> MAAAVAMETDDAGNRLRFQLELEFVQCLANPNYLNFLAQRGYFKDKAFVNYLKYLLYWKEPEYAKYLKYPQCLHMLELLQYEHFRKELVNAQCAK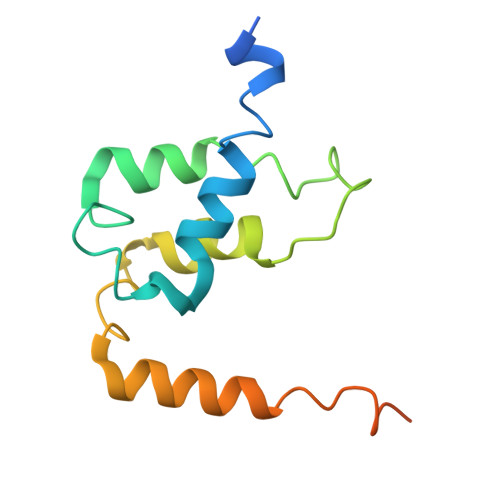FIDEQQILHWQHYSRKRVRLQQALAEQQQQNNTAGK N,N-dibenzyl-N~5~-[N-(methylcarbamoyl)carbamimidoyl]-N~2~-{[5-({[(E)-(quinolin-4-ylmethylidene)amino]oxy}methyl)-1H-1,2,3-triazol-1-yl]acetyl}-L-ornithinamide | C37 H41 N11 O4 | 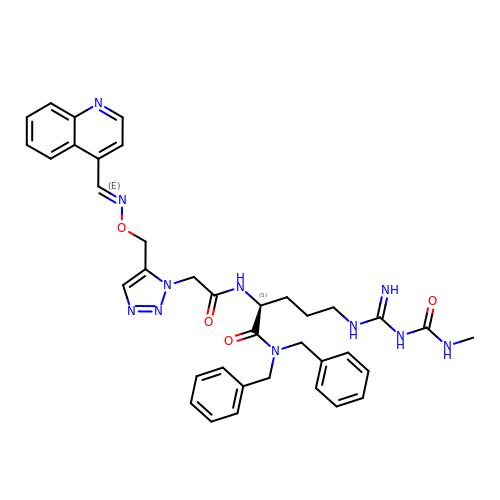YASCYEPUKAYRJI-IPZIAFNWSA-N>SNAMTTSDTTDRSQDGVPPLSFHQEFLCMFDSGNDGADVGPFGPMYHIVGAWRLTGGIDEETLREALGDVVVRHEALRTSLVREGGTHRPEILPAGPAALEVRDLGDVDESERVRRGEELLNEVESTGLSVRELPLLRAVLGRFDQKDAVLVLIAHHTAADAWAMHVIARDLLNLYAARRGNPVPPLPEPAQHAEFARWEREAAEAPRVAVSKEFWRKRLQGARIIGLETDIPRSAGLPKGTAWQRFAVRGELADAVVEFSRAAKCSPFMTMFAAYQVLLHRRTGELDITVPTFSGGRNNSRFEDTVGSFINFLPLRTDLSGCASFREVVLRTRTTC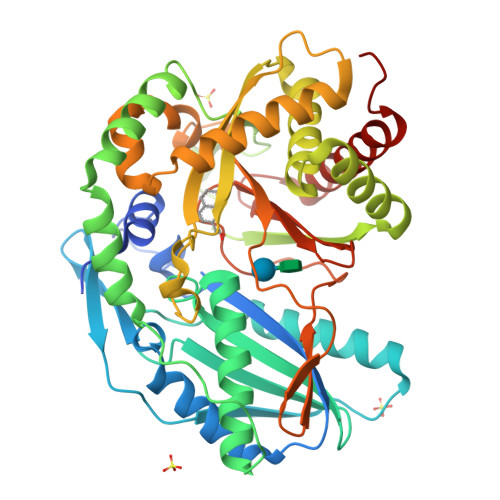GEAFTHELPFSRLIPEVPELMASAASDNHQISVFQAVHAPASEGPEQAGDLTYSKIWERQLSQAEGSDIPDGVLWSIHIDPSGSMAGSLGYNTNRFKDETMAAFLADYLDVLENAVARPDAPFTS[2x]> SGRGEAETRECIYYNANWELERTNQSGLERCEGEQDKRL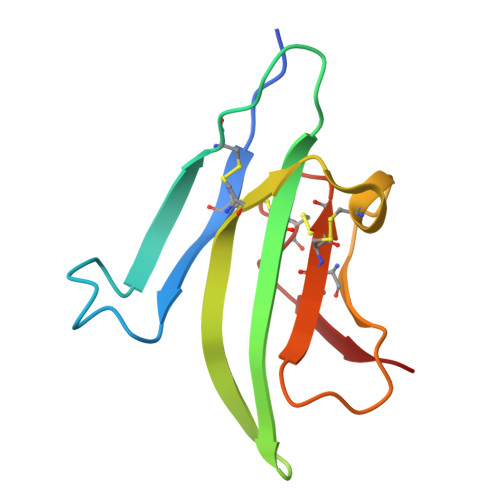HCYASWRNSSGTIELVKKGCWLDDFNCYDRQECVATEENPQVYFCCCEGNFCNERFTHLP> GSHGGSMSGSFELSVQDLNDLLSDGSGCYSLPSQPCNEVTPRIYVGNASVAQDIPKLQKLGITHVLNAAEGRSFMHVNTNANFYKDSGITYLGIKANDTQEFNLSAYFERAADFIDQALAQKNGRVLVHCREGYSRSPTLVIAYLMMRQKMDVKSALSIVRQNREIGPNDGFLAQLCQLNDRLAKE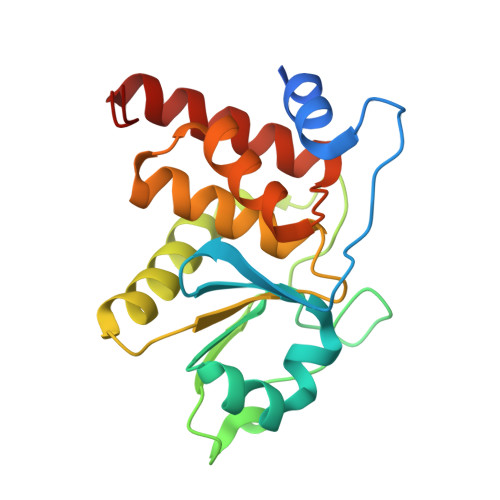GKLKP>MKRFFNRFYLDTGIIADPSQRSLASRVSAFLVQGAVAFSLLGTIGVDTSPLIAAAGVTGATIGFACKDFGTNFVASIVLSGQQSIRTGNLVCIGTGLNVVKGKVVDWDTRY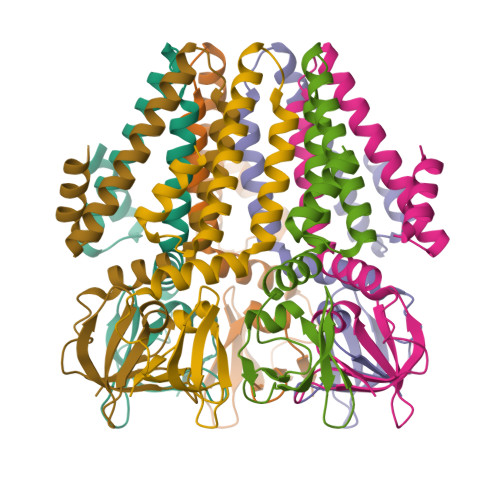LYLRSSEGHLLHVPNNMVLNSVVTWEQEKKQNPHETDLPKQDVVKAPGDNAAKQSNSLEVLFQ[7x]>[2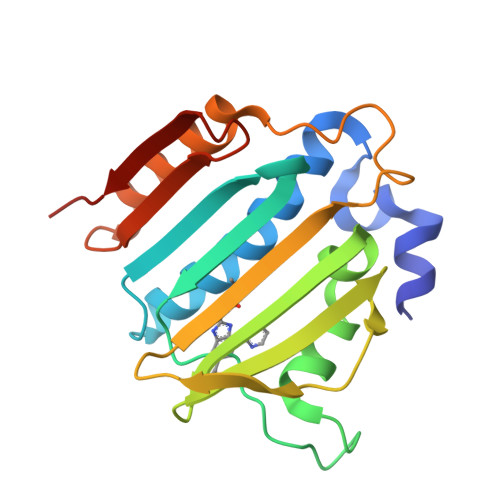x]MEGLEAVRKRPGMYIGSTSERGLHHLVWEIVDNSIDEALAGYANQIEVVIEKDNWIKVTDNGRGIPVDIQEKMGRPAVEVILTSSVVNALSQDLEVYVHRNETIYHQAYKKGVPQFDLKEVGTTDKTGTVIRFKADGEIFTETTVYNYETLQQRIRELAFLNKGIQITLRDERDEENVREDSYHYEG Two plasmid-encoded dihydrofolate reductase (DHFR) isoforms, DfrA1 and DfrA5, that give rise to high levels of resistance in Gram-negative bacteria were structurally and biochemically characterized to reveal the mechanism of TMP resistance and to support phylogenic groupings for drug development against antibiotic resistant pathogens. TMP is a selective inhibitor of bacterial dihydrofolate reductase (DHFR), which catalyzes the NADPH-dependent reduction of dihydrofolate (DHF) to tetrahydrofolate (THF), a necessary step for the recycling of reduced folate cofactors. Trimethoprim resistance in Enterobacteriaceae occurs almost exclusively through the acquisition of plasmid-associated dfr genes that encode intrinsically insensitive DHFR enzymes. Expectedly, all three enzymes form the stereotypical DHFR fold with an eight-stranded β-sheet, four α-helices (B, C, E, and F) and three catalytic loops (the Met20, F-G, and G-H loops).

Like TMP, the PLA binding mode is dictated through hydrogen bonding with Asp27EcDHFR or Glu28DfrA1/DfrA5, and the propargyl linker forms π–π interactions with Phe31. However, unlike TMP, the bicyclic moiety forms van der Waals contacts with helix C (residues 43–50). In the DfrA5:NADPH:UCP1223 structure, UCP1223 makes van der Waals contacts with Gln29, Met51, Leu54, and the bicyclic moiety is swung out of the pocket, exposing the highly polar benzylamine to bulk solvent. Interestingly, the UCP1223 had a distinctly stabilizing effect across all three enzymes, agreeing well with our crystal structures where a racemic mixture of this ligand is likely adopting different binding poses for an optimal configuration. Critically, unlike TMP, the PLAs preferentially form the ternary complex with NADPH in their respective DfrA complexes. When superimposed, both structures of DfrA1 and DfrA5 complexed with UCP1223 and UCP1228 show a clear density for NADPH. The PLA scaffold is able to accommodate the noted structural changes imparted by the D27E substitution allowing for conformational flexibility that favors ternary complex formation.

>[2x]MKVSLMAAKAKNGVIGCGPHIPWSAKGEQLLFKALTYNQWLLVGRKTFESMGALPNRKYAVVTRSAWTADNDNVIVFPSIEEAMYGLAELTDHVIVSGGGEIYRETLPMASTLHISTIDIEPEGDVFFPNIPNTFEVVFEQHFSSNINYCYQIWQKG We use bacteriophage φ6, a member of the Cystoviridae family, as a model system to study the assembly of a complicated multi-shelled virus. The inner T=1 shell, composed of protein P1, forms a dodecahedral polymerase complex (PC) harbouring the three viral dsRNA segments (S, M, and L), the viral polymerase P2, the hexameric packaging protein P4, and the assembly cofactor P7. The expanded PC is covered by a layer of P8, forming the outer T=13 shell. Here we present the structure of φ6 NC to near-atomic resolution using electron cryomicroscopy and single particle analysis.

In φ6, the vertices are occupied by the P4 packaging hexamer. The six-fold symmetry of the P4 hexamer and five-fold symmetry of the icosahedral vertex beneath creates a symmetry mismatch, so that the structure of P4 cannot be resolved using conventional icosahedral reconstruction. To address this we applied the localized reconstruction method17 to P4 hexamers. Local areas corresponding to P4 hexamers were extracted from the NC images and reconstructed as single particles with six-fold symmetry (‘P4 hexamer reconstruction') or without any symmetry (‘NC vertex reconstruction'). This allowed a low-resolution structure of the P4 hexamer to be determined in situ. However, in earlier low-resolution cryo-EM reconstructions, the P4 hexamers appeared to float on top of the five-fold vertexes of the P1 shell23 and the connections between these symmetry-mismatched components have remained unresolved. Binding of up to five of the six flexible C-terminal tails of P4 provides an elegant solution to the symmetry mismatch. These tails are likely to be disordered in solution and to order only upon binding to P1 during assembly. Our modelling experiments also showed that six P1A–P1B dimers per P4 would create steric clashes. It is thus likely that each P4 grabs five and not more P1A–P1B dimers.

>[6x]MPIVVTQAHIDRVGIAADLLDASPVSLQVLGRPTAINTVVIKTYIAAVMELASKQGGSLAGVDIRPSVLLKDTAIFTKPKAKSADVESDVDVLDTGIYSVPGLARKPVTHRWPSEGIYSGVTALMGATGSGKSITLNEKLRPDVLIRWGEVAEAYDELDTAVHISTLDEMLIVCIGLGALGFNVAVDSVRPLLFRLKGAASAGGIVAVFYSLLTDISNLFTQYDCSVVMVVNPMVDAEKIEYVFGQVMASTVGAILCADGNVSRTMFRTNKGRIFNGAAPLAADTHMPSMDRPTSMKALDHTSIASVAP OKADAIC 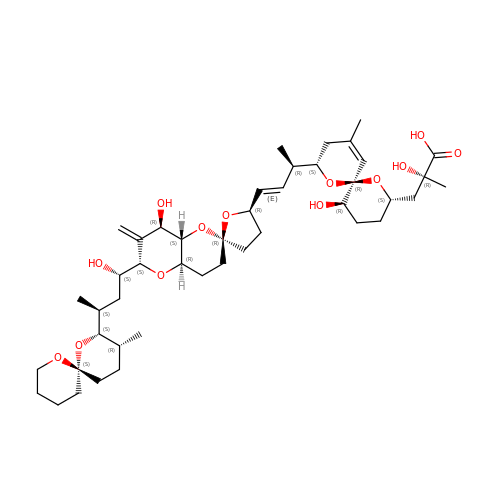ACID | C44 H68 O13 | QNDVLZJODHBUFM-WFXQOWMNSA-N4-[[3-(5-fluoranyl-2-oxidanyl-phenyl)phenyl]sulfonylamino]-2-oxidanyl-benzoic 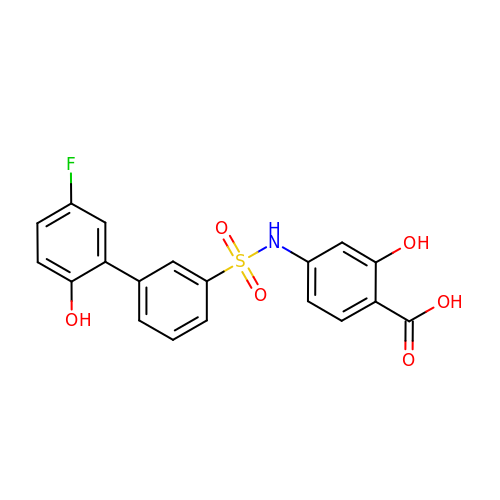acid | C19 H14 F N O6 S | DDVUKRHRMBDQTD-UHFFFAOYSA-N> MSYYHHHHHHLESTSLYKKAGFMSLQRIVRVSLEHPTSAVCVAGVETLVDIYGSVPEGTEMFEVYGTPGVDIYISPNMERGRERADTRRWRFDATLEIIVVMNSPSNDLNDSHVQISYHSSHEPLPLAYAVLYLTCVDISLDCDLNCEGRQDRNFVDKRQWVWGPSGYGGILLVNCDRDDPSCDVQDNCDQHVHCLQDLEDMSVMVLRTQGPAALFDDHKLVLHTSSYDAKRAQVFHICGPEDVCEAYRHVLGQDKVSYEVPRLHGDEERFFVEGLSFPDAGF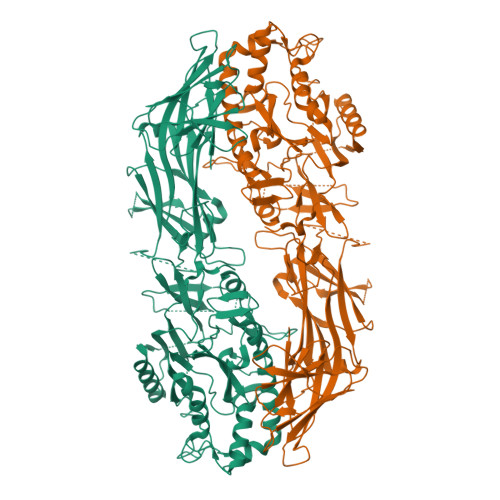TGLISFHVTLLDDSNEDFSASPIFTDTVVFRVAPWIMTPSTLPPLEVYVCRVRNNTCFVDAVAELARKAGCKLTICPQAENRNDRWIQDEMELGYVQAPHKTLPVVFDSPRNGELQDFPYKRILGPDFGYVTREPRDRSVSGLDSFGNLEVSPPVVANGKEYPLGRILIGGNLPGSSGRRVTQVVRDFLHAQKVQPPVELFVDWLAVGHVDEFLSFVPAPDGKGFRMLLASPGACFKLFQEKQKCGHGRALLFQGVVDDEQVKTISINQVLSNKDLINYNKFVQSCIDWNREVLKRELGLAECDIIDIPQLFKTERKKATAFFPDLVNMLVLGKHLGIPKPFGPIINGCCCLEEKVRSLLEPLGLHCTFIDDFTPYHMLHGEVHCGTNVCRKPFSFKWWNMVP> LEADKCKEREEKIILVSSANEIDVRPCPLNPNEHKGTITWYKDDSKTPVSTEQASRIHQHKEKLWFVPAKVEDSGHYYCVVRNSSYCLRIKISAKFVENEPNLCYNAQAIFKQKLPVAGDGGLVCPYMEFFKNENNELPKLQWYKDCKPLLLDNIHFSGVKDRLIVMNVAEKHRGNYTCHASYTYLGKQYPITRVIEFITLEENKPTRPVIVSPANETMEVDLGSQIQ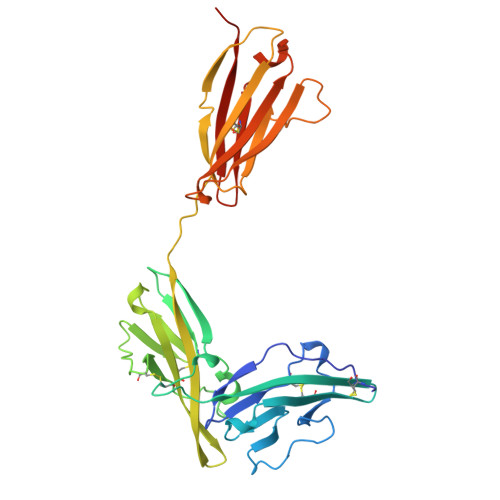LICNVTGQLSDIAYWKWNGSVIDEDDPVLGEDYYSVENPANKRRSTLITVLNISEIESRFYKHPFTCFAKNTHGIDAAYIQLIYPVTNFQK> AQSVPYGVSQIKAPALHSQGYTGSNVKVAVIDSGIDSSHPDLKVAGGASMVPSETPNFQDDNSHGTHVAGTVAALNNSIGVLGVAPSSALYAVKVLGDAGSGQYSWIINGIEWAIANNMDVINMSLGGPSGSAALKAAVDKAVASGVVVVAAAGNEGSTGSSSTVGYPGKYPSVIAVGAVDSSNQRASFSSVGPELDVMAPGVSIQSTLPGNKYGAYNGTSMASPHVAGAAALILSKH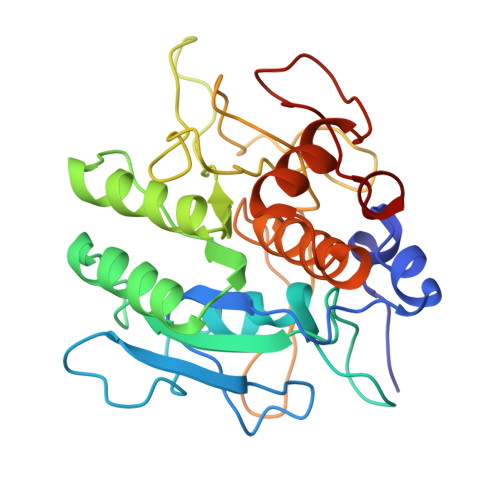PNWTNTQVRSSLQNTTTKLGDSFYYGKGLINVQAAAQ Histone deacetylases (HDACs) regulate the acetylation state of lysine residues of histones as well as other protein substrates, and therefore play a pivotal role in many cellular processes. Specifically targeting two or more distinct HDACs can also be beneficial, but this presents a particular challenge when those two HDACs belong to different isozyme classes with different structural requirements for efficient binding (the Zn2+‐dependent HDACs are grouped into Class I (HDACs 1,2,3,8), Class IIa (HDACs 4,5,7,9), Class IIb (HDACs 6,10) and Class IV (HDAC11)). We report the synthesis and evaluation of a class of selective multitarget agents for the inhibition of HDAC6, HDAC8, and HDAC10. Hybridization of the two inhibitor structures resulted in dihydroxamic acids with benzyl‐indole and ‐indazole core motifs.

KGaAParallel to our biochemical evaluation, we attempted to co‐crystallize the dual inhibitors with Danio rerio (zebrafish) HDAC10,32 where we had introduced A24E and D94A substitutions to more closely resemble the human HDAC10 active site. However, due to the rigidity and bulk of 3a there are significant local structural changes in the active site. Specifically, the 310 helix containing the P23(E,A)CE motif that protrudes into the active site shifts, on average, by 1.4 Å (maximum shift=1.9 Å). However, the current structure reveals that this motif can shift to accommodate the binding of certain bulky inhibitors. Zinc coordination by the ionized hydroxamate group of 3a is achieved by a mixture of two different monodentate binding modes. The hydroxamate of the major conformer (67 % occupancy) coordinates to zinc through the N−O− group (O−Zn2+ separation=2.1 Å). At first glance, the hydroxamate group of the minor conformer of 3a (33 % occupancy) appears to coordinate to Zn2+ in a manner similar to that observed for bidentate hydroxamate‐zinc interactions as observed in other HDAC10‐inhibitor complexes. Thus, inner sphere Zn2+ coordination is achieved solely by the hydroxamate N−O−group (O−Zn2+ separation=2.4 Å). The phenyl ring of 3a makes favorable offset π stacking interactions in an aromatic crevice defined by F146 and W205, as well as the Zn2+ binding residue H176. The A24E substitution was made to “humanize” the active site of zebrafish HDAC10, so the packing interaction between E24 and the indole ring of 3a is presumably important for binding to human HDAC10.

> AASGSALIFDEEMSRYKLLWTDPECEIEVPERLTVSYEALRTHGLAQRCKAVPVRQATEQEILLAHSEEYLEAVKQTPGMNVEELMAFSKKYNAVYFHQNIYHCAKLAAGATLQLVDSVMKREVRNGMALVRPPGHHSQRSAANGFCVFNNVAFAALYAKKNYNLNRILIVDWDVHHGQGIQYCFEEDPSVLYFSWHRYEHQSFWPNLPESDYSSVGKGKGSGFNINLPWNKVGMTNSDYLAAFFHVLLPVAYEFDPELVIVSAGFDSAIGDPEGEMCALPEIFAHLTHLLMPLAAGKMCVVLEGGYNLTSLGQSVCQTVHSLLGDPTPRISGLGTACDSALESIQNVRNVQSSYWSSFKHLAQSETNPKRPRLDATNGGPKESSEPASESNPKKTAQDIVWPEPLKRMPASVRTVVVPPPGVELTLPKNCQHSGDISESTAKEVQRIRDKHFHDLTDQNILRSLGNIISVLDRMMRSDEVCNGCVVVSDLSVSVQCALQHALTEPAERVLVVYVGDGELPVKTNDGKVFLVQICTKETEDKCVNRLTLCLREGESLTAGFMQALLGLILPVAYEFNPALVLGIVEETAAKTRLMRVWGHMTCLIQGLARGRMLTLLQGYDKDLLELTVSALSGASISPLGPLRAPKPEDVEMMEKQRQRLQERWGLLRCTVSESW>[4x]MAHHHHHHVDDDDKPGPALYEENALKGKIDDPNSYVPDAVQEAYKN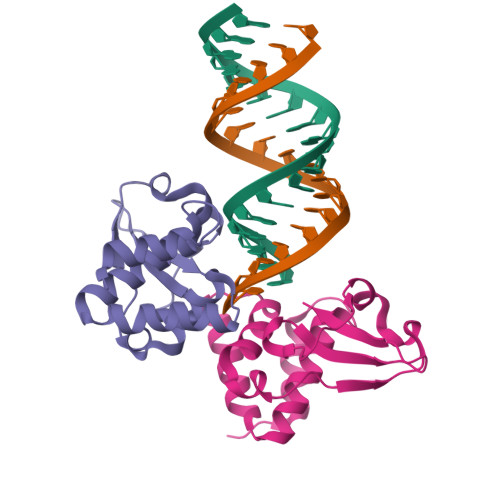LDSTSTLTEENFGKPYISAKDLKEIMYDHLPGFGTAFHQLVQVICKIGKDNNLLDTIHAEFQASLADGDSPQCALIQITKRVPIFQDVPPPIIHIRSRGDIPRACQKSLRPAPPSPKIDRGWVCLFKMQDGKTLGLKI>[2x]AAVTQSPRNKVAVTGEKVTLSC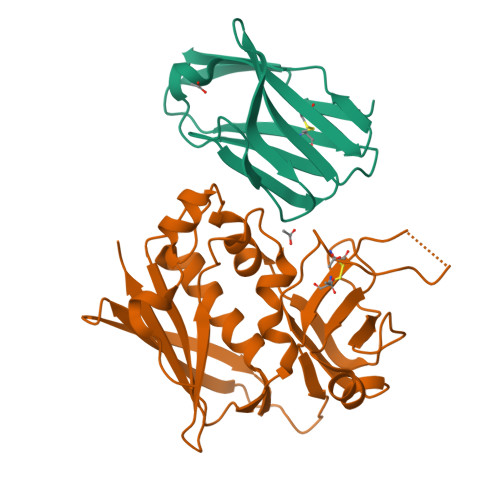QQTNNHNNMYWYRQDTGHGLRLIHYSYGAGSTEKGDIPDGYKASRPSQEQFSLILESATPSQTSVYFCASGGGGTLYFGAGTRLSVL;>QPDPKLDELNKVSDYKSNKGTMGNVMNLYMSPPVEGRGVINSRQFLSHDLIFPIEYKSYNEVKTELENTELANNYKGKKVDIFGVPYFYTCIIPKSEPDINQNFGGCCMYGGLTFNSSENERDKLITVQVTIDNRQSLGFTITTNKNMVTIQELDYKARHWLTKEKKLYEFDGSAFESGYIKFTEKNNTSFWFDLFPKKELVPFVPYKFLNIYGDNKVVDSKSIKMEVFLNTHHHHHHH[2x]Tailed double-stranded DNA (dsDNA) bacteriophages and their eukaryotic counterparts, such as herpesviruses, possess a dodecameric portal at a unique vertex of the capsid; this portal serves as a channel for DNA packaging during viral assembly and delivery. The portal interacts with multiple copies of a scaffolding protein (SP) to form a nucleation complex, which initiates the assembly of the major capsid protein (i.e., coat protein) and other minor proteins into a procapsid. The P22 procapsid consists of an icosahedral coat comprising 415 coat protein (gene product [gp] 5) subunits, a dodecameric ring comprising portal protein (gp1) subunits located at a unique capsid vertex, and an internal core comprising approximately 250–300 SP (gp8) subunits and 3 ejection proteins. In this study, we present the structure of the SP gp8 in complex with the dodecameric portal in the P22 procapsid at subnanometer resolution.

When the density map of the portal and domes at a resolution of 15 Å was displayed at 1.9 times the standard deviation, the side view of the GOF nodules revealed that the outer dome contained three neighboring four-blade windmill-like structures. The four blades of each windmill-like structure in the outer dome were connected to the inner dome through a column, with one blade contributed by a side nodule. To confirm this notion, we performed local reconstruction of the windmill-like structure. The results indicated that each windmill-like structure comprised four gp8 subunits, constituting a gp8 tetramer. Each blade comprised a base dimer. The outermost part of each blade was not part of the gp8 tetramer but was instead contributed by the base domain of a neighboring gp8 subunit. The gp8 tetramer was stabilized through a four-helix bundle formed by the four-column domains. The tetramers interacted with other gp8 subunits in neighboring tetramers through electrostatic interactions between the base domains. Local reconstruction of the top region of the outer dome revealed that this region comprised gp8 tetramers. The SP tetramer primarily forms through interactions of the C-terminal region (residues 122–136) within the column domain; this explains why a recombinant SP fragment (residues 141–303) does not form tetramers.

>[8x]MEPTTEIQATEDLTLSGDHAAASADSLVVDNANDNAGQEEGFEIVLKDDETAPKQDPAKNAEFARRRIERKRQRELEQQMEAVKRGELPESLRVNPDLPPQPDINAYLSEEGLAKYDYDNSRALAAFNAANTEWLMKAQDARSNAVAEQGRKTQEFTQQSAQYVEAARKHYDAAEKLNIPDYQEKEDAFMQLVPPAVGADIMRLFPEKSAALMYHLGANPEKARQLLAMDGQSALIELTRLSERLTLKPRGKQISSAPPADQPITGDVSAANKDAIRKQMDAAASKGDVETYRKLKAKLKGIR>[2x]MAITADDIAVQYPIPTYRFIVTLGDEQVPFTSASGLDINFDTIEYRDGTGNWFKMPGQRQAPNITLSKGVFPGKNAMYEWINAIQLNQVEKKDIMISLTNEAGTEVLVSWNVSNAFPTSLTSPSFDATSNEIAVQQITLMADRVTIQTA;> MTVTTTYPGVYLSEDAVSSFSVNSAATAVPLFAYDSENTNTINKPIQVFRNWAEFTVEYPTPLEDAFYTSLSLWFMHGGGKCYLVNEANIADAVAQYDDITLIVAAGTDTTTYTAFTTVVGQGYRIFGLFDGPKEKIAGTAKPDEVMEEYPTSPFGAVFYPWGTLASGAAVPPSAIAAASITQTDRTRGVWKAPANQAVNGVTPAFAVSDDFQGKYNQGKALNMIRTFS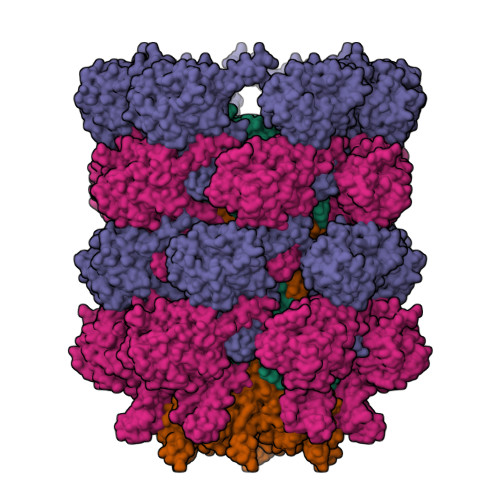GQGTVVWGARTLEDSDNWRYIPVRRLFNAVERDIQKSLNKLVFEPNSQPTWQRVKAAVDSYLHSLWQQGALAGNTPADAWFVQVGKDLTMTQEEINQGKMIIKIGLAAVRPAEFIILQFSQDIAQ;> MATVTSVPGVYIEEDASPAMSVSASATAVPLFVARFTPLKPELAGVITRIGSWLDYTILFDSNVPSSARVTVSSTAVEPSPEFDALETASSKATTTYTYQIDDTEVVDPTASVALRLYFQNGGGPCYLYPLEKADDNGPLAALPDLIDEVGEITLLASPDPDETYRTAVYGALAASLDQHKGYFLLADSVNGDAPSAVGGSAQVAVYYPNVEVPHTRKLDDAEVAIDGYLDDEGKAVTTLAALRVVNTEFAGEIAQSLSGDLSAPLSLPPSALIAGVYGKTDGERGVWKAPANVVLNGVSDVSVRVTNEQQAELNPKGINVIRHFSDRGLVVWGSRTQKDDDDWRYIPVRRLFDAAERDIKKALQPMVFEPNSQLTWKRVQTAIDNYLYRLWQQGALAGNKAEEAYFVRVGKGITMTQDEINQGKMIIQVGMAAVRPAEFIILKFTQDMSQ>MYKLVPQIDTR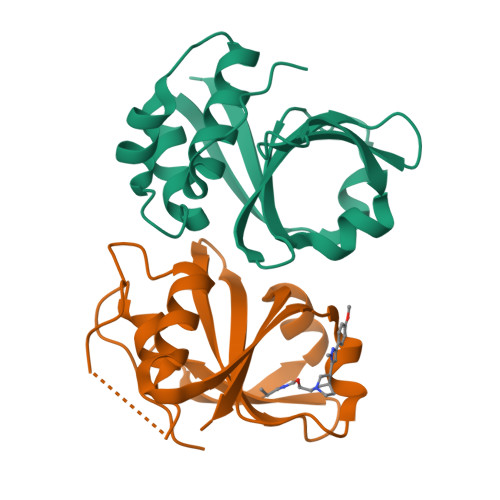DCGPAVLASVAKHYGSNYSIAYLRELSKTNKQGTTALGIVEAAKKLGFETRSIKADMTLFDYNDLTYPFIVHVIKGKRLQHYYVVYGSQNNQLIIGDPDPSVKVTRMSKERFQSEWTGLAIFLAPQPNYKPHKGEHHHHHH[2x]>[2x]MGSDKIHHHHHHMNVLALDTSQRIRIGLRKGEDLFEISYTGEKKHAEILPVVVKKLLDELDLKVKDLDVVGVGIGPGGLTGLRVGIATVVGLVSPYDIPVAPLNSFEMTAK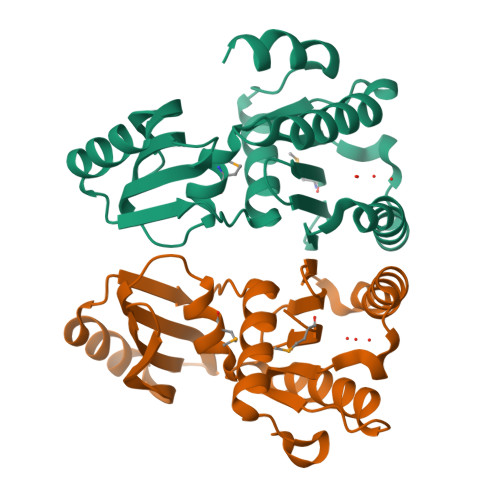SCPADGVVLVARRARKGYHYCAVYLKDKGLNPLKEPSVVSDEELEEITKEFSPKIVLKDDLLISPAVLVEESERLFREKKTIHYYEIEPLYLQKSIAELNWEKKKRG5-{2-[2-(2,4-dioxo-3,4-dihydropyrimidin-1(2H)-yl)ethoxy]phenoxy}-7-fluoronaphthalene-2-carbonitrile 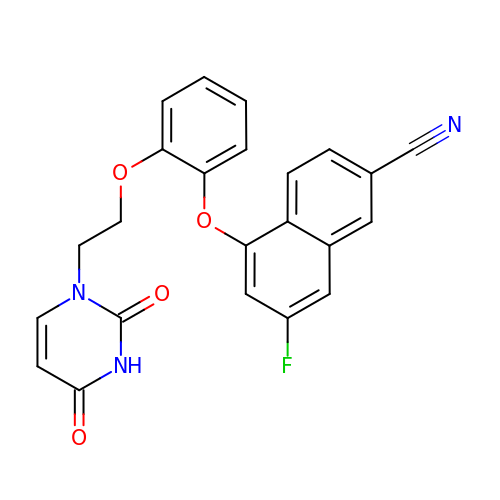| C23 H16 F N3 O4 | CZZSYVLCOGCXLL-UHFFFAOYSA-N>MAFNPAPKAVQENHHVDYVIRFNYGDIDTPEAIKKFEVLLLELSEVGLQTEVRQGDENSLFVFVRAASKKKLKRAVYQSRVRDWLYGVRNTEPEPASSAKPQSEAERLLVIYHLITVPKAEGGAGITPRHGEWKNVDAIFPLHDEETNRQCMREWSKKTFLSTEDLDRIRNTFGEHVGFYFAFLQSYFRFLMFPAAFGFSCWLLLGSFSIIYTVVNCLWCIVFIEYWKRQEEDLSCRWQTKGVSAVHEKRAEFKPEKEIRDESTGEVRGVFPATKRMYRQLLQVPFALLAAVALGAIIATCFAIEIFISEVYNGPLKGYLVFIPTILVSALIPTMSAVLLTVATKLNDYENYETQDAYKVALTQKIFVVNFITSYLPIILTAFVYVPFASRIVPYLDVFHLTVRPFVSKEHAIKARTEFSINPDRLRKQVIYFTVTAQIVGFALETIVPFVKQRVFREYKEYTKKQHAKAEPGNGAGEKKTVSLGDDEDEARFLTRVRNEAELEDYDVTDDLREMCIQFGYLALFSPVWPLVPVSFLINNWVELRSDFFKICVECKRPWPQRADTIGPWLDSLGFLSWVGSITSSALVYMFSNGHEGPNGEPTTIRCWALLLTIFFSEHLYLIVRYAVRSALAKLEPPNTRRERIERFMMRKRYLDTVLSAESDDDADEVKGVVSSIPPSEITRESLEQDARDWSKQGTDPTERFWMRQRGWKESAEVGLSLITKAKGDETKKQQ[2x]

TMEM16 scramblases dissipate the plasma membrane lipid asymmetry to activate multiple eukaryotic cellular pathways. The TMEM16 superfamily is comprised of Cl- channels and dual function scramblases/non-selective ion channels. Our results show afTMEM16 thins the membrane to enable scrambling and that an open hydrophilic pathway is not a structural requirement to allow rapid transbilayer movement of lipids. Scrambling by the TMEM16’s is modulated by two signals, binding of Ca2+ facilitates opening of the groove while the properties of the membrane determine whether the scramblase can thin the membrane enough to enable lipid flipping.

In contrast, in C14 lipids scrambling in 0 Ca2+ is ~30% of that seen in saturating Ca2+ so that if scrambling requires groove opening, we expect that a significant portion of particles would adopt a Ca2+-free open-groove conformation. Analysis of a C14/0 Ca2+ afTMEM16 dataset yields only classes with a closed groove, Cα r.m.s.d. ~0.9 Å to C18/0 Ca2+, the highest of which reached 3.3 Å average resolution. Thus, in 0 Ca2+ changing from C18 to C14 lipids induces a ~8-fold increase in scrambling activity that is not accompanied by a concomitant increase in the probability of opening of the groove. This suggests that the basal, Ca2+ independent activity is due to closed-groove scrambling. In the C14/0 Ca2+ map, thickness at the closed pathway qualitatively approaches that at the open pathway of the C18/Ca2+ map, consistent with enhanced scrambling. In the three datasets for apo afTMEM16 (C18/0 Ca2+, C14/0 Ca2+ and DA/EA in 0.5 mM Ca2+) we could resolve 4–9 lipids per monomer, all localized near the dimer interface in positions closely resembling those seen in C18/Ca2+ structure, supporting the notion that these lipids interact strongly with the protein. No lipids could be resolved near the closed pathway in these structures. In thinner membranes, closed-groove scrambling is enhanced allowing for lipid transport in the absence of Ca2+.>MESPEEPGASMDENYFVNYTFKDRSHSGRVAQGIMKLCLEEELFADVTISVEGREFQLHRLVLSAQSCFFRSMFTSNLKEAHNRVIVLQDVSESVFQLLVDYIYHGTVKLRAEELQEIYEVSDMYQLTSLFEECSRFLARTVQVGNCLQVMWLADRHSDPELYTAAKHCAKTHLAQLQNTEEFLHLPHRLLTDIISDGVPCSQNPTEAIEAWINFNKEEREAFAESLRTSLKEIGENVHIYLIGKESSRTHSLAVSLHCAEDDSISVSGQNSLCHQITAACKHGGDLYVVGGSIPRPRRMWKCNNATVDWEWCAPLPRDRLQHTLVSVPGKDAIYSLGGKTLQDTLSNAVIYYRVGDNVWTETTQLEVAVSGAAGANLNGIIYLLGGEENDLDFFTKPSRLIQCFDTETDKCHVKPYVLPFAGRMHAAVHKDLVFIVAEGDSLVCYNPLLDSFTRLCLPEAWSSAPSLWKIASCNGSIYVFRDRYKKGDANTYKLDPATSAVTVTRGIKVLLTNLQFVLA[2x];>[2x]MAYSQGGGKKKVCYYYDGDIGNYYYGQGHPMKPHRIRMTHNLLLNYGLYRKMEIYRPHKATAEEMTKYHSDEYIKFLRSIRPDNMSEYSKQMQRFNVGEDCPVFDGLFEFCQLSTGGSVAGAVKLNRQQTDMAVNWAGGLHHAKKSEASGFCYVNDIVLAILELLKYHQRVLYIDIDIHHGDGVEEAFYTTDRVMTVSFHKYGEYFPGTGDLRDIGAGKGKYYAVNFPMRDGIDDESYGQIFKPIISKVMEMYQPSAVVLQCGADSLSGDRLGCFNLTVKGHAKCVEVVKTFNLPLLMLGGGGYTIRNVARCWTYETAVALDCEIPNELPYNDYFEYFGPDFKLHISPSNMTNQNTPEYMEKIKQRLFENLRMLPHAPGVQMQAIPEDAVHEDSGDEDGEDPDKRISIRASDKRIACDEEFSDSEDEGEGGRRNVADHKKGAKKARIEEDKKETEDKKTDVKEEDKSKDNSGEKTDTKGTKSEQLSNP

Kelch repeat and BTB domain-containing protein 4 (KBTBD4) is the substrate receptor of a cullin3-dependent E3 ligase complex (CRL3KBTBD4). Recurrent indel mutations in the Kelch domain of the KBTBD4 E3 ligase rewire epigenetic programs for stemness in medulloblastoma by recruiting LSD1-CoREST-HDAC1/2 complexes as neo-substrates for ubiquitination and degradation. UM171, an investigational drug for haematopoietic stem cell transplantation, was found to degrade LSD1-CoREST-HDAC1/2 complexes in a wild-type KBTBD4-dependent manner, suggesting a potential common mode of action. The mutant and drug-induced complexes adopt similar structural assemblies requiring both Kelch domains in the KBTBD4 dimer for each HDAC2 interaction.

The best map at 2.7 Å was obtained for the higher affinity sample mixing KBTBD4R313PRR and CoREST1NT2-HDAC2. The modelled structure revealed a KBTBD4R313PRR dimer engaging two HDAC2 molecules in C2 symmetry (2:2 stoichiometry, Fig. 4a, b, although a rare 2D class with one HDAC2 (2:1) was also observed, Supplementary Fig. 4). The mutant KBTBD4R313PRR was resolved to near full length, consisting of BTB, BACK and Kelch domains, whereas only the histone deacetylase domain could be modelled from the full-length HDAC2 construct; density was also lacking for its associated CoREST1NT2 subunit. Each HDAC2 subunit in the 2:2 model makes direct contacts with both Kelch domains in the KBTBD4R313PRR dimer by engaging the mutant BC II loop from one chain (site 1) and the BC IV loop (blade IV, site 2) from the other. Most importantly, the indel mutation extends the length of BC II and shifts the position of KBTBD4 R312, a non-mutated residue, by 5.9 Å to the tip of the loop. This structural alteration allows the R312 side chain to insert into the catalytic pocket of HDAC2 to within 5.7 Å of the catalytic Zn2+ ion, which natively binds to acetyl-lysines in histone H3 and H4 tails. In addition, the R312 side chain is sandwiched between HDAC2 F151 and F206 to form cation-π interactions. Additional cation-π interaction is observed between KBTBD4R313PRR R314 and HDAC2 Y205 close to the exit of the HDAC2 catalytic pocket. Here, KBTBD4R313PRR L408, F410 and F411 from the BC IV loop form extended hydrophobic interactions with an HDAC2 cleft that features Y202, L212, P228, Y359 and I363. Additionally, the binding is stabilised by a salt bridge between KBTBD4R313PRR D409 and HDAC2 R230.>[2x]GHMKISRETLHQLIENKLCQAGLKREHAATVAEVLVYADARGIHSHGAVRVEYYAERISKGGTNREPEFRLEETGPCSAILHADNAAGQVAAKMGMEHAIKTAQQNGVAVVGISRMGHSGAISYFVQQAARAGFIGISMCQSDPMVVPFGGAEIYYGTNPLAFAAPGEGDEILTFDMATTVQAWGKVLDARSRNMSIPDTWAVDKNGVPTTDPFAVHALLPAAGPKGYGLMMMIDVLSGVLLGLPFGRQVSSMYDDLHAGRNLGQLHIVINPNFFSSSELFRQHLSQTMRELNAITPAPGFNQVYYPGQDQDIKQRKAAVEGIEIVDDIYQYLISDALYNTSYETKNPFAQ

In this study, we determined the crystal structures of E. coli (S)-ureidoglycolate dehydrogenase AllD, which forms oxalurate in the presence of NAD+. This structure represents a metabolic branch point enzyme during (S)-ureidoglycolate utilization, which is the end product of purine catabolism common to plants, as well as some bacteria and fungi. (S)-Ureidoglycolate dehydrogenase AllD belongs to one of eight clades of l-sulfolactate dehydrogenase-like superfamily. The dimeric structure observed in the asymmetric unit represents the functional unit of AllD, consistent with size-exclusion chromatography, in which AllD eluted as a dimer.

However, we were able to identify the binding site of glyoxylate in the vicinity of NADH when a crystal was soaked with oxalurate. In particular, a NADH cofactor is located at the site identical to that in the binary complex. The formation of glyoxylate could have occurred through the spontaneous degradation of oxalurate under our experimental conditions, and its binding site could provide the binding mode of (S)-ureidoglycolate substrate. The electron density map for glyoxylate was unambiguous in subunit A, but not in subunit B. The planar molecule glyoxylate is 4.0–5.0 Å over the B-face of the nicotinamide, but with a perpendicular orientation to it. Specifically, the carboxylate group interacts with Arg48 within a distance of 3.4 Å, and its position is further stabilized by hydrogen bonds at a distance of 3.1–3.4 Å to His116, Ser140, and the amino group of the nicotinamide ring. In contrast, the aldehyde carbonyl oxygen orients toward the opposite direction of the nicotimamide ring, and is within 3.9 Å of the nearby residues Asp141 and Met251. In the ternary complex, further changes were not observed, except for Asp141, whose side chain rotated as much as 3.9 Å toward glyoxylate. However, the aldehyde carbon of glyoxylate is too distant from the C4 atom of NADH (about 6.0 Å) for the proposed hydride transfer reaction. Therefore, the binding mode of glyoxylate is apparently different from that of the substrate, although the glyoxylate moiety provides general information about the substrate binding site.> QELQELRRELE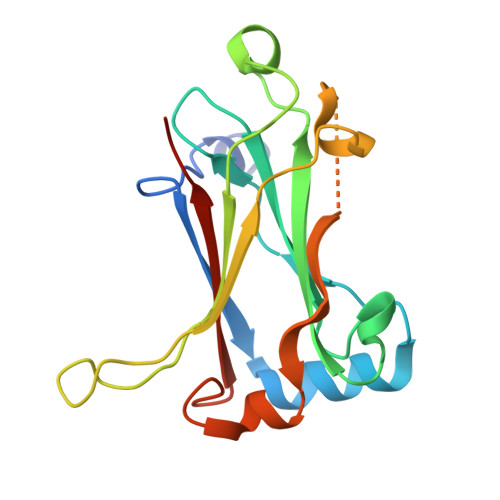ELSVGSDGVLIWKIGSYGRRLQEAKAKPNLECFSPAFYTHKYGYKLQVSAFLNGNGSGEGTHLSLYIRVLPGAFDNLLEWPFARRVTFSLLDQSDPGLAKPQHVTETFHPDPNWKNFQKPGTWRGSLDESSLGFGYPKFISHQDIRKRNYVRDDAVFIRAAVELPRKILS>MAEKVLVTGGAGYIGSHTVLELLEAGYLPVVIDNFHNAFRGGGSLPESLRRVQELTGRSVEFEEMDILDQGALQRLFKKYSFMAVIHFAGLKAMGESVQKPL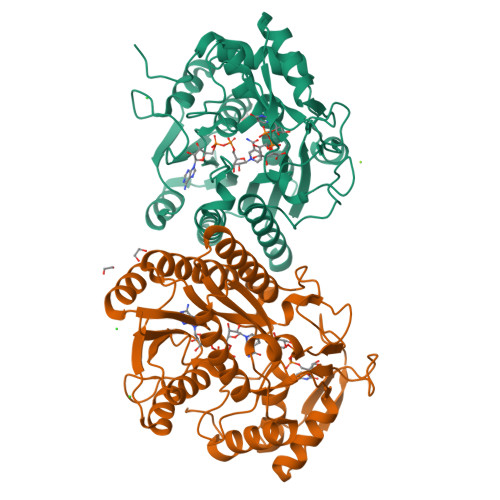DYYRVNLTGTIQLLEIMKAHGVKNLVFSSSATVYGNPQYLPLDEAHPTGGCTNPYGKSKFFIEEMIRDLCQADKTWNVVLLRYFNPTGAHASGCIGEDPQGIPNNLMPYVSQVAIGRREALNVFGNDYDTEDGTGVRDYIHVVDLAKGHIAALRKLKEQCGCRIYNLGTGTGYSVLQMVQAMEKASGKKIPYKVVARREGDVAACYANPSLAQEELGWTAALGLDRMCEDLWRWQKQNPSGFGTQA[2x]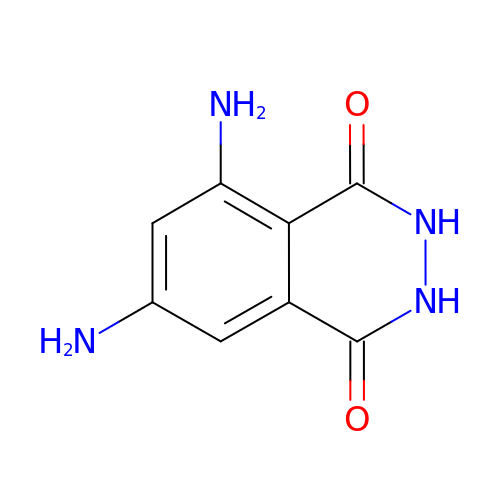3,5-DIAMINOPHTHALHYDRAZIDE | C8 H8 N4 O2 | BAOICLZZDLLDRL-UHFFFAOYSA-N>[2x]SKKRQWALEDFEIGRPLGKGKFGNVYLAREKQSKFILALKVLFKAQLEKAGVEHQLRREVEIQSHLRHPNILRLYGYFHDATRVYLILEYAPLGTVYRELQKLSKFDEQRTATYITELANALSYCHSKRVIHRDIKPENLLLGSAGELKIADFGWSVHAPSSRRDTLCGTLDYLPPEMIEGR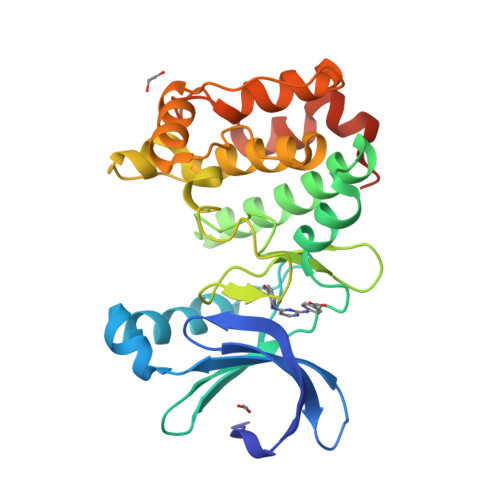MHDEKVDLWSLGVLCYEFLVGKPPFEANTYQETYKRISRVEFTFPDFVTEGARDLISRLLKHNPSQRPMLREVLEHPWITANSSKPSNCQNKESASK>[2x]GSEFQNKNFRAPQSEAIGILYKLIETGSKHKNMYDHTEITTDSLLALLGSEKVKIIDVRSADAYNGWRMRGEVRGGHIKGAKSLPAKWLTDPEWLNIVRFKQIRPEDAIVLYGYTPEECEQTATRFKENGYNNVSVFHRFHPDWTGNDAFPMDRLEQYNRLVPAEWVNGLISG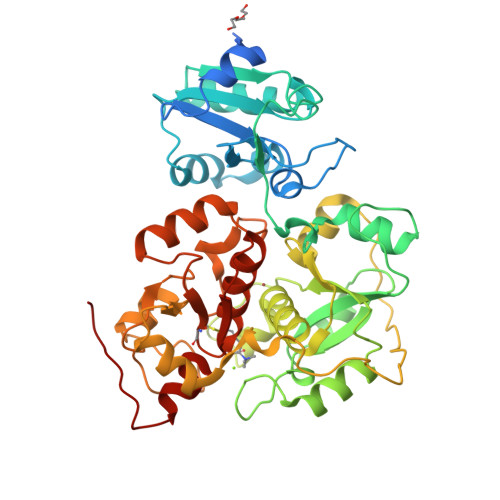EEIPEYDNDTFIVCHAHYRNRDAYLSGHIPGATDMDTLALESPETWNRRTPEELKKALEEHGITASTTVVLYGKFMHPDNADEFPGSAAGHIGAIRLAFIMMYAGVEDVRVLNGGYQSWTDAGFAISKDDVPKTTVPEFGAPIPSRPEFAVDIDEAKEMLQSEDSDLVCVRSYPEYIGEVSGFNYIKKKGRIPGAIFAECGSDAYHMENYRNHDHTTREYHEIEDIWAKSGIIPKKHLAFYCGTGWRGSEAWFNALLMGWPRVSVYDGGWFEWSNDPENPYETGVPK>[3x]MRCIGISNRDFVEGVSGGSWVDIVLEHGSCVTTMAKNKPTLDFELIKTEAKHPATLRKYCIEAKLTNTTTASRCPTQGEPSLNEEQDKRFVCKHSMVDRGWGNGCGLFGKGGIVTCAMFTCKKNMEGKVVQPENLEYTIVITPHSGEENAVGNDTGKHGKEIKVTPQSSITEAELTGYGTVTMECSPRTGLDFNEMVLLQMENKAWLVHRQWFLDLPLPWLPGADTQGSNWIQKETLVTFKNPHAKKQDVVVLGSQEGAMHTALTGATEIQMSSGNLLFTGHLKCRLRMDKLQLKGMSYSMCTGKFKVVKEIAETQHGTIVIRVQYEGDGSPCKIPFEIMDLEKRHVLGRLITVNPIVTEKDSPVNIEAEPPFGDSYIIIGVEPGQLKLSWFKKGSSIGQMFETTMRGAKRMAILGDTAWDFGSLGGVFTSIGKALHQVFGAIYGAAFSGVSWTMKILIGVVITWIGMNSRSTSLSVSLVLVGVVTLYLGVMVQA;>[3x]SVALVPHVGMGLETRTETWMSSEGAWKHAQRIETWVLRHPGFTIMAAILAYTIGTTYFQRVLIFILLTAVAPSMT

Flaviviruses are positive-strand RNA viruses with enveloped virus particles. The E protein is responsible for attachment to target cells and mediates fusion between the viral and cellular membranes during entry. During the transit of the virion through the secretory pathway, acidification and cleavage of prM into pr and M induce large rearrangements of the spike at the viral surface, ultimately resulting in antiparallel homodimers arranged in a characteristic herringbone pattern. The C-terminal domain forms a stem consisting of three membrane-proximal helices (E-H1, E-H2 and E-H3) and two transmembrane helices (E-T1 and E-T2).

Our best reconstruction based on the BinJV platform has been determined for bDENV-2 to a resolution of 2.5 Å. Density is present for ~150 water molecules for each M–E heterodimer. Improved modelling in the stem region revealed discrete electron densities that were not accounted for in our model. The bifurcated envelopes can accommodate a phosphatidylethanolamine molecule (site 1) and a phosphoceramide molecule (site 2), respectively, with the fatty acid tails pointing towards the membrane. The two sites are located on either side of E-H1 in the stem of E. Site 1 is closer to the membrane and is largely open with sufficient space for another lipid between E-H1 and E-H3 as suggested at low-density thresholds. Site 2 consists of a narrow gap between E-H1, E-H3 and the top of the C-terminal transmembrane helix E-T2, and a wider cavity accommodating the head group of the putative phosphoceramide molecule located underneath the ectodomain of E and near the stem of M. Using site-directed mutagenesis, we show that most contact residues are essential for the formation of viable virus. Specifically, residues Arg411 in E-H1 and Trp420 in E-H2 are essential in site 1 and residues His437, Gly441, Tyr444, Phe448 in E-H3 and Leu489 in E-T2 in site 2. Thus, in the immature virions, both sites are absent indicating that the pocket factors are not acquired during biogenesis of the glycoproteins and early steps of assembly.>[4x]MLTVDLSGKKALVMGVTNQRSLGFAIAAKLKEAGAEVALSYQAERLRPEAEKLAEALGGALLFRADVTQDEELDALFAGVKEAFGGLDYLVHAIAFAPREAMEGRYIDTRRQDWLLALEVSA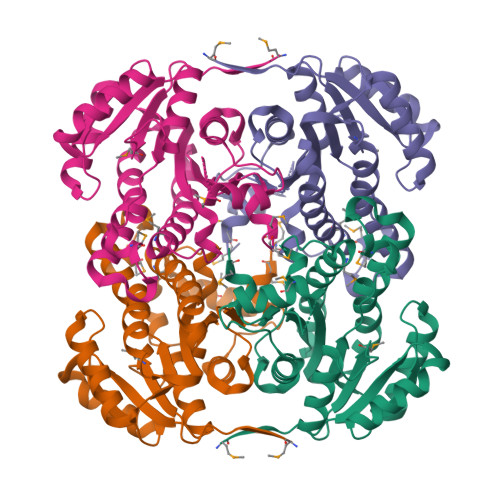YSLVAVARRAEPLLREGGGIVTLTYYASEKVVPKYNVMAIAKAALEASVRYLAYELGPKGVRVNAISAGPVRTVAARSIPGFTKMYDRVAQTAPLRRNITQEEVGNLGLFLLSPLASGITGEVVYVDAGYHIMGMELEG> MAAGKLKKEQQNQSAERESADTGKVNDEDEEHLYGNIDDYKHLIQDEEYDDEDVPHDLQLSEDEYNSERDSSLLAEFSDYGEISEDDEEDFMNAIREASNFKVKKKKKNDKGKSYGRQRKERVLDPEVAQLLSQANEAFVRNDLQVAERLFNEVIKKDARNFAAYETLGDIYQLQGRLNDCCNSWFLAAHLNASDWEFWKIVAILSADLDHVRQAIYCFSRVISLNPMEWESIYRRSMLYKKTGQLARALDGFQRLYMYNPYDANILRELAILYVDYDRIEDSIELYMKVFNANVERREAILAALENALDSSDEESAAEGEDADEKEPLEQDEDRQMFPDINWKKIDAKYKCIPFDWSSLNILAELFLKLAVSEVDGIKTIKKCARWIQRRESQTFWDHVPDDSEFDNRRFKNSTFDSLLAAEKEKSYNIPIDIRVRLGLLRLNTDNLVEALNHFQCLYDETFSDVADLYFEAATALTRAEKYKEAIDFFTPLLSLEEWRTTDVFKPLARCYKEIESYETAKEFYELAIKSEPDDLDIRVSLAEVYYRLNDPETFKHMLVDVVEMRKHQVDETLHRISNEKSSNDTSDISSKPLLEDSKFRTFRKKKRTPYDAERERIERERRITAKVVDKYEKMKKFELNSGLNEAKQASIWINTVSELVDIFSSVKNFFMKSRSRKFVGILRRTKKFNTELDFQIERLSKLAEGDSVFEGPLMEERVTLTSATELRGLSYEQWFELFMELSLVIAKYQSVEDGLSVVETAQEVNVFFQDPERVKMMKFVKLAIVLQMDDEEELAENLRGLLNQFQFNRKVLQVFMYSLCRGPSSLNILSSTIQQKFFLRQLKAF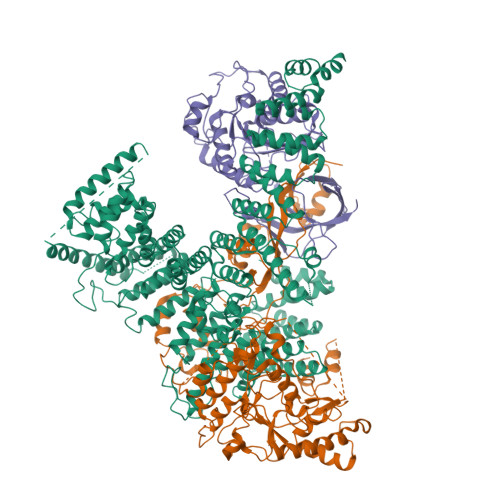DSCRYNTEVNGQASITNKEVYNPNKKSSPYLYYIYAVLLYSSRGFLSALQYLTRLEEDIPDDPMVNLLMGLSHIHRAMQRLTAQRHFQIFHGLRYLYRYHKIRKSLYTDLEKQEADYNLGRAFHLIGLVSIAIEYYNRVLENYDDGKLKKHAAYNSIIIYQQSGNVELADHLMEKYLSIRSGG;> MHHHHHHENLYFQSMPVEEPLATLSSIPDSSADQAPPLIADEFTLDLPRIPSLELPLNVSTKHSSIQKAIKMCGGIEKVKEAFKEHGPIESQHGLQLYLNDDTDSDGSKSYFNEHPVIGKRVPFRDESVILKVTMPKGTLSKNNNSVKDSIKSLKDSNKLRVTPVSIVDNTIKFREMSDFQIKLDNVPSAREFKSSFGSLEWNNFKSFVNSVPDNDSQPQENIGNLILDRSVKIPSTDFQLPPPPKLSMVGFPLLYKYKANPFAKKKKNGVTEVKGTYIKNYQLFVHDLSDKTVIPSQAHEQVLYDFEVAKKTKVYPGTKSDSKFYESLEECLKILRELFARRPIWVKRHLDGIVPKKIHHTMKIALALISYRFTMGPWRNTYIKFGIDPRSSVEYAQYQTEYFKIERKLLSSPIVKKNVPKPPPLVFESDTPGGIDSRFKFDGKRIPWYLMLQIDLLIGEPNIAEVFHNVEYLDKANELTGWFKELDLVKIRRIVKYELGCMVQGNYEYNKYKLKYFKTMLFVKESMVPENKNSEEGMGVNTNKDADGDINMDAGSQMSSNAIEEDKGIAAGDDFDDNGAITEEPDDAALENEEMDTDQNLKVPASIDDDVDDVDADEEEQESFDVKTASFQDIINKIAKLDPKTAETMKSELKGFVDEVDLXXXXXXXXXXXXXXXXXXXXXX;> MVVNTIYIARHGYRSNWLPEGPYPDPLTGIDSDVPLAEHGVQQAKELAHYLLSLDNQPEAAFASPFYRCLETVQPIAKLLEIPVYLERGIGEWYRPDRKPVIPVPAGYEILSKFFPGVISQEWDSTLTPNEKGETEQEMYMRFKKFWPLFIERVEKEYPNVECILLVTHAASKIALGMSLLGYDNPRMSLNENGDKIRSGSCSLDKYEILKKSYDTIDETDDQTSFTYIPFSDRKWVLTMNGNTEFLSSGEEMNWNFDCVAEAGSDADIKKRQMTKKTSSPIPEADDQTEVETVYISVDIPSGNYKERTEIAKSAILQYSGLETDAPLFRIGNRLYEGSWERLVGTELAFPNAAHVHKKTAGLLSPTEENETTNAGQSKGSSTANDPNIQIQEEDVGLPDSTNTSRDHTGDKEEVQSEKIYRIKERIVLSNVRPM>[2x]GHMTDSEFFHQRF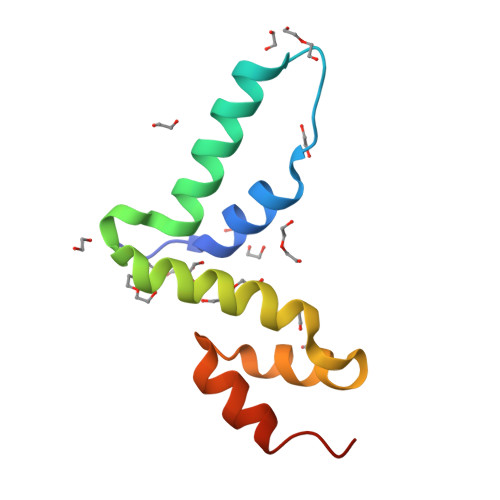RNLIYVEFVGPRKTLIKLRNLCLDWLQPETRTKEEIIELLVLEQYLTIIPEKLKPWVRAKKPENCEKLVTLLENYKEMYQP>MSETVLSQESAAKKTQFKVIDTDIHHDIASVDDLVPYLSDHWKRYITEYNWKPIKTTPFHQVRSGTKYRGDSFGESKRPPGSDFELLKKQLLDEHEITYGVLGGWFHEATVATGWFEFAAARAAAYNDYTIEQWLNKDERLLGSITIPADPVAAVREIDRVGPHPQMVQVMMSIGNFAWGDPRFHPIFEAAERHGLAIGMHLSADITFQGGEFLRYYVAWRAAHPQAYMTQVISLITNGVFDKYPNLKVALIEGGFEWVPFMMNRMDAAYKGLRQETPWVKRMPSDYFRDNMRFSTQPWHDISAKHFLDIIDMMGSDKMLMFSTDYPHWDFDAPKRTLPPKISDDLKNKILYENARELYNL[4x]

Dinuclear monooxygenases mediate challenging C–H bond oxidation reactions throughout nature. The protein components of AibH1H2 stem from a largely uncharacterized structural superfamily, PF04909, containing over 100,000 unique proteins that can individually function as either carboxylases, hydratases, hydrolases, or monooxygenases. Representatives of the latter enzyme class—collectively defined here as “amidohydrolase-related dinuclear oxygenases” (AROs)—include PtmU313 and AibH2,9,15 which employ dinuclear cofactors with different metal identities. Herein we utilize this “guilt by association” strategy to identify four candidate AROs that can each harbor redox-active dinuclear active sites. Each of the four candidate AROs can harbor redox-active diiron cofactors.

The genomic neighborhoods of candidate AROs stemming from Litorilinea aerophila (A0A540VG95, referred to as SfbO), Afipia carboxidovorans (B6JH23), Cytobacillus firmus (W7L2Y2), and Geobacillus strain Y412MC10 (D3EI84) intimate disparate physiological functions. Each of these proteins was fused to an N-terminal His6 tag, recombinantly expressed in Escherichia coli, and purified as soluble protein preparations. For initial studies, the expression medium was supplemented with additional FeII sources to ensure the formation of an intact dinuclear active site. Aerobic samples of these Fe2-metalated proteins were found to exhibit moderately intense UV/vis features centered near ∼350 nm, consistent with charge transfer bands classically associated with diferric FeIII–OHx–FeIII motifs. These features were diminished upon anaerobic addition of ∼1.2 equiv of sodium dithionite (DT) and returned following reexposure of these samples to air.>GAAAMSNLLTLHHSLPALPADATSDEVRKNLMDVFRDRPAFSEHTWEMLLSVCRSWAAWCKLNNRKWFPAEPEDVRDYLLHLQARGLAVKTIQQHLCRLNMLHRRSGLPRPSDSNAVSLVMRRIRKENVDAGERTKQALAFERTDFDQVRSLMENSDRCQDIRNLAFLGVAYNTLLRIAEIARIRVKDISRTDGGRMLIHIGRTKTLVSTAGVEKALSLGVTKLVERWISVSGVADDPNNYLFCRVRRYGVAAPSA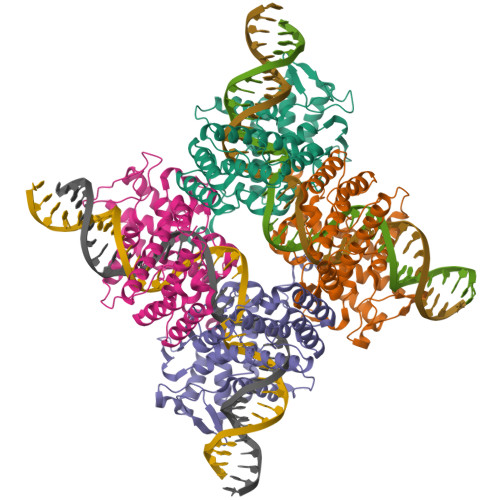TSQLSTYALQRIFEATHRLIYGAKDDSGQRYLAWSGHSARVGAARDMARAGVSIPEIMQAGGWTTVNSVMNFIRNLDSETGAMVRLLED[4x]> XKKGACES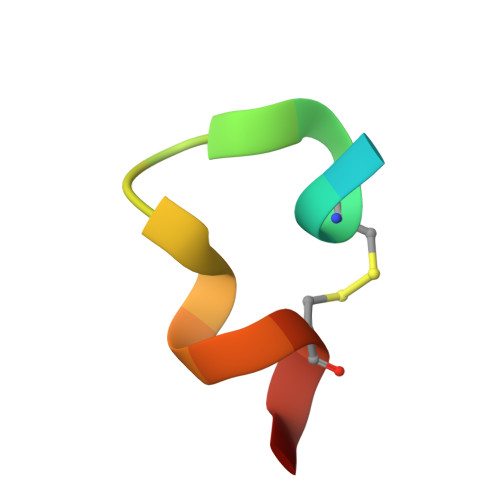PEWQWLCAAX> IVGGQECKDGECPWQALLINEENEGFCG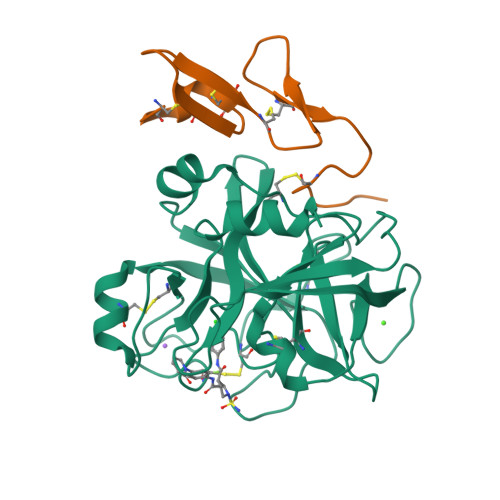GTILSEFYILTAAHCLYQAKRFKVRVGDRNTEQEEGGEAVHEVEVVIKHNRFTKETYDFDIAVLRLKTPITFRMNVAPACLPERDWAESTLMTQKTGIVSGFGRTHEKGRQSTRLKMLEVPYVDRNSCKLSSSFIITQNMFCAGYDTKQEDACQGDSGGPHVTRFKDTYFVTGIVSWGEGCARKGKYGIYTKVTAFLKWIDRSMKTRGLPKAK;> RKLCSLDNGDCDQFCHEEQNSVVCSCARGYTLADNGKACIPTGPYPCGKQTLERR>[4x]MELHILE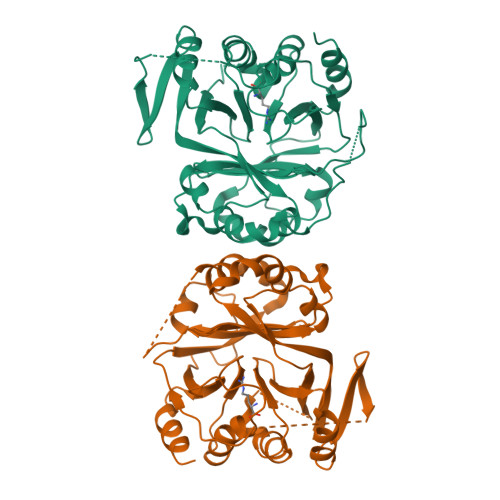HRVRVLSVARPGLWLYTHPLIKLLFLPRRSRCKFFSLTETPEDYTLMVDEEGFKELPPSEFLQVAEATWLVLNVSSHSGAAVQAAGVTKIARSVIAPLAEHHVSVLMLSTYQTDFILVREQDLSVVIHTLAQEFDIYREVGGEPVPVTRDDSSNGFPRTQHGPSPTVHPIQSPQNRFCVLTLDPETLPAIATTLIDVLFYSHSTPKEAASSSPEPSSITFFAFSLIEGYISIVMDAETQKKFPSDLLLTSSSGELWRMVRIGGQPLGFDECGIVAQIAGPLAAADISAYYISTFNFDHALVPEDGIGSVIEVLQRRQEGLASLEHHHHHH> MSLPAHLQQTFSPEEIQFIVENEPIKIFPRITTRQKIRGDDRGTGNHTRWQLITTDDKALNNMVAMRSTEVVLWIALLLKQQSKCSIVAPQWLTTKELDRKIQYEKTHPDRFSELPWNWLVLARILFNKAKDDFHD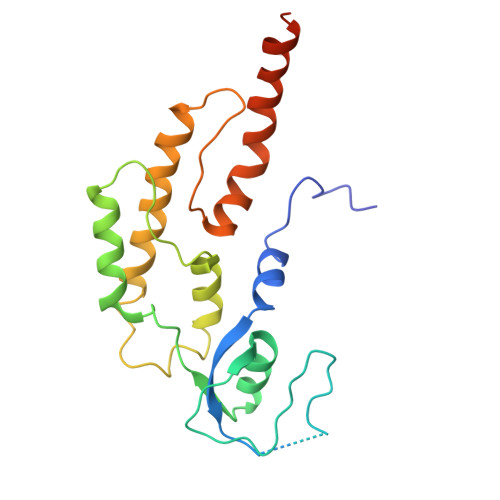PIHELRGKIQDLREIRQIKVLKGLKYLNESHLQLDNLSLLEINELRPFITEIMDKLREIHTASLTAGTENDEEEFNI>ANPLYQKHIISINDLSRDDLNLVLATAAKLKANPQPELLKHKVIASCFFEASTRTRLSFQTSMHRLGASVVGFSDSANTSLGKKGETLADTISVISTYVDAIVMRHPQEGAARLATEFSGNVPVLNAGDGSNQHPTQTLLDLFTIQQTEGRLDNLHVAMVGDLKYGRTVHSLTQALAKFDGNRFYFIAPDALAMPEYILDMLDEKGIAWSLHSSIEEVMAEVDILYMTRVQKERLDPSEYANVKAQFVLRASDLHNAKANMKVLHPLPRVDEIATDVDKTPHAWYFQQAGNGIFARQALLALVLNRDLVL[2x];>[2x]MTHDNKLGVEAIKRGTVIDHIPAQIGFKLLSLFKLTETDQRITIGLNL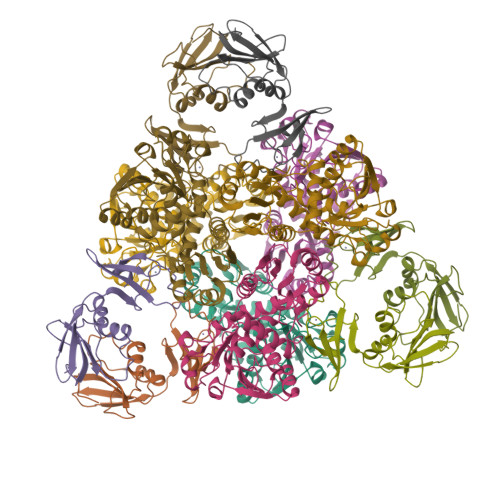PSGEMGRKDLIKIENTFLSEDQVDQLALYAPQATVNRIDNYEVVGKSRPSLPERIDNVLVCPNSNCISHAEPVSSSFAVRKRANDIALKCKYCEKEFSHNVVLAN> MILRASVLSALLLVGLGAAPKHSVSANDKRMQDNLVSVIEKQTNKKVRILEIKPLKSSQDLKMVVIEDPDTKYNIPLVVSKDGNLIIGLSNIFFSNKSDDVQLVAETNQKVQALNATQQNSAKLNAIFNEIPADYAIELPSTNAANKDKILYIVSDPMCPHCQKELTKLRDHLKENTVRMVVVGWLGVNSAKKAALIQE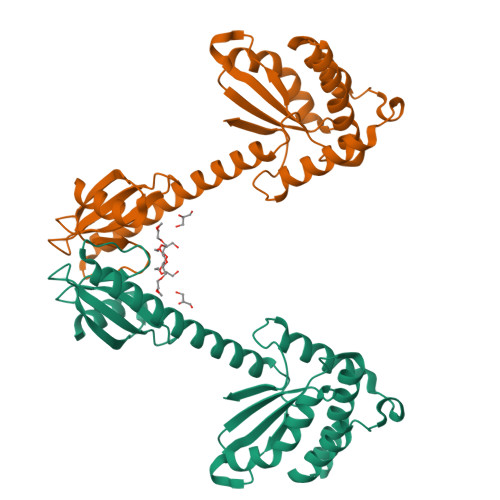EMAKARARGASVEDKISILEKIYSTQYDINAQKEPEDLRTKVENTTKKIFESGVIKGVPFLYHYKALEHHHHHH> XUGCUGGCUAA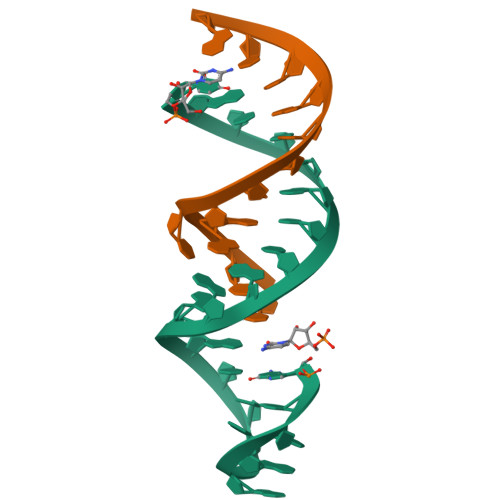GGGCCGAAAGX;> CUAUGCCUGCUG> IEMKP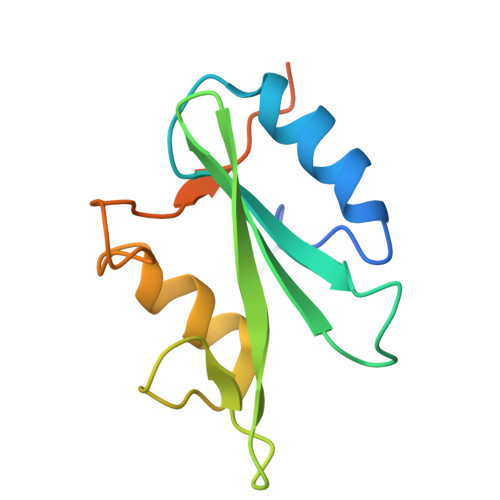HPWFFGKIPRAKAEEMLSKQRHDGAFLIRESESAPGDFSLSVKFGNDVQHFKVLRDGAGKYFLWVVKFNSLNELVDYHRSTSVSRNQQIFLRDIEQVPQQPTYVQAHHHHHH>RALEVERTVSLAEVYAGLPKDNGPFSLAQEIDKLVSQGSGSAGSGNNNLAFGAGTDTKTSLQASVSFADLKIREDYPASLGKIRRIKQISVTLPALLGPYQDVQAILSYGDKAGLANGCEALAVSHGMNDSGQFQLDFNDGKFLPFEGIAIDQGTLTLSFPNASMPEKGKQATMLKTLNDIILHIRYTIK[5x];> MQNSQTFSVTELSLPKGGGAITGMGEALTPAGPDGMAALSLPLPISAGRGYAPSLTLNYNSGTGNSPFGLGWDCGVMAIRRRTSTGVPNYDETDTFLGPEGEVLVVALNEAGQADIRSESSLQGINLGATFTVTCYRSRLESHFNRLEYWQPQTTGATDFWLIYSPDGQVHLLGKNPQARISNPLNVNQTAQWLLEASISSHSEQIYYQYRAEDEAGCETDELAAHPSATVQRYLQTVHYGNLTASDVFPTLNGDDPLKSGWMFCLVFDYGERKNSLSEMPLFKATGNWLCRKDRFSRYEYGFELRTRRLCRQILMFHRLQTLSGQAKGDDEPALVSRLILDYDENAMVSTLVSVRRVGHEDNNTVTALPPLELAYQPFEPEQTALWQSMDVLANFNTIQRWQLLDLKGEGVPGILYQDRNGWWYRSAQRQAGEEMNAVTWGKMQLLPITPAVQDNASLMDINGDGQLDWVITGPGLRGYHSQHPDGSWTRFTPLHALPIEYSHPRAQLADLMGAGLSDLVLIGPKSVRLYVNNRDGFTEGRDVVQSGDITLPLPGADARKLVAFSDVLGSGQAHLVEVSATQVTCWPNLGHGRFGQPIVLPGFSQSAASFNPDRVHLADLDGSGPADLIYVHADRLDIFSNESGNGFAKPFTLSFPDGLRFDDTCQLQVADVQGLGVVSLILSVPHMAPHHWRCDLTNAKPWLLSETNNNMGANHTLHYRSSVQFWLDEKAAALATGQTPVCYLPFPVHTLWQTETEDEISGNKLVTTLRYAHGAWDGREREFRGFGYVEQTDSHQLAQGNAPERTPPALTKSWYATGLPAVDNALSAGYWRGDKQAFAGFTPRFTLWKEGKDVPLTPEDDHNLYWLNRALKGQPLRSELYGLDGSAQQQIPYTVTESRPQVRQLQDGATVSPVLWASVVESRSYHYERIISDPQCNQ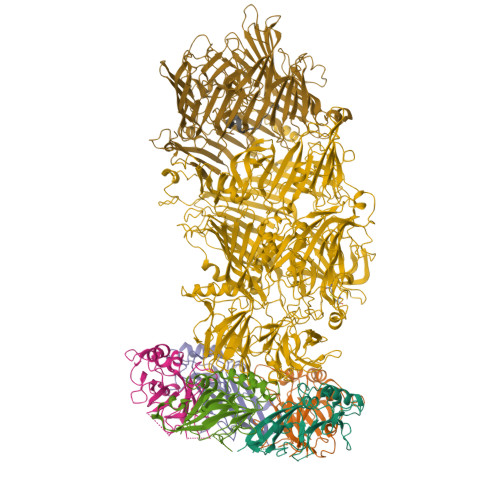DITLSSDLFGQPLKQVSVQYPRRNKPTTNPYPDTLPDTLFASSYDDQQQLLRLTCRQSSWHHLIGNELRVLGLPDGTRSDAFTYDAKQVPVDGLNLETLCAENSLIADDKPREYLNQQRTFYTDGKNQTPLKTPTRQALIAFTETAVLTESLLSAFDGGITPDELPGILTQAGYQQEPYLFPRTGENKVWVARQGYTDYGTEAQFWRPVAQRNSLLTGKMTLKWDTHYCVITQTQDAAGLTVSANYDWRFLTPTQLTDINDNVHLITLDALGRPVTQRFWGIESGVATGYSSSEEKPFSPPNDIDTAINLTGPLPVAQCLVYAPDSWMPLFSQETFNTLTQEEQETLRDSRIITEDWRICALTRRRWLQSQKISTPLVKLLTNSIGLPPHNLTLTTDRYDRDSEQQIRQQVAFSDGFGRLLQASVRHEAGEAWQRNQDGSLVTKVENTKTRWAVTGRTEYDNKGQTIRTYQPYFLNDWRYVSDDSARKEAYADTHIYDPIGREIRVITAKGWLRQSQYFPWFTVSEDENDTAADALV;> MSSYNSAIDQKTPSIKVLDNRKLNVRTLEYLRTQADENSDELITFYEFNIPGFQVKSTDPRKNKNQSGPNFIRVFNLAGQVLREESVDAGRTITLNDIESRPVLIINATGVRQNHRYEDNTLPGRLLAITEQVQAGEKTTERLIWAGNTPQEKDYNLAGQCVRHYDTAGLTQLNSLSLAGVVLSQSQQLLVDDKNADWTGEDQSLWQQKLSSDVYTTQNKADATGALLTQTDAKGNIQRLAYDVAGQLKGCWLTLKGQAEQVIIKSLTYSAAGQKLREEHGNGVITEYSYEPETQRLIGIATRRPSDAKVLQDLRYQYDPVGNVINIRNDAEATRFWRNQKVVPENSYTYDSLYQLISATGREMANIGQQNNQLPSPALPSDNNTYTNYTRSYSYDHSGNLTQIRHSSPATQNNYTVAITLSNRSNRGVLSTLTTDPNQVDTLFDAGGHQTSLLPGQTLIWTPRGELKQVNNGPGNEWYRYDSNGMRQLKVSEQPTQNTTQQQRVIYLPGLELRTTQSNATTTEELHVITLGEAGRAQVRVLHWESGKPEDVNNNQLRYSYDNLIGSSQLELDNQGQIISEEEYYPFGGTALWAANSQTEASYKTIRYSGKERDATGLYYYGYRYYQPWAGRWLSADPAGTIDGLNLYRMVRNNPVSLQDENGL;> APEKGKYTKEVNFFDE Here, we report a family of bacterial actins of unknown function, conserved among the Verrucomicrobiota phylum, which assembles into a unique tubular structure in the presence of ATP. We identified a family of actin homologs, most closely related to MamK (25 to 30% sequence identity) but present in non-magnetotacic bacteria, and therefore presumably with a distinct function. Sequence analysis confirms that it possesses the conserved residues for ATP binding and hydrolysis, and structure prediction confirmed that it likely adopts an actin-like fold. 2d classification suggested that it adopts a rail tracks-like architecture, consisting of two strands rotating on their individual axis (Inset). This prompted us to name this family the Bacterial elongated entwined Rail-like protein (BeeR).

We next used cryo-EM to determine the structure of the BeeR filament, to 3.1 Å resolution. This revealed that it adopts a three-stranded, parallel, right-handed, staggered filament architecture. The diameter of this filament, at ~80 Å, is significantly larger than most other actin-like proteins, and it includes a ~25 Å-wide cavity at its core, responsible for its rail track-like appearance by negative-stain EM. BeeR possesses the canonical actin domains Ia, Ib, IIa, and IIb, with the nucleotide buried between domains Ib and IIb. The longitudinal interface along strands is largely similar to other actin-like filaments, with domains Ib and IIb making extensive contacts with domains IIa of the subunit above. The cross-strand contacts in the BeeR filament are distinct to that of other actin-like filaments. Each protomer interacts with two consecutive subunits of the adjacent strand, as shown on Fig. 2C. Contacts with the top subunit are minimal, with an interface area of ~35 Å2, and consist of a hydrogen bond network between Arg 157 of one subunit and Thr 307 and Gln 310 in the adjacent subunit. In contrast, the contact with the bottom subunit is extensive, forming a contact surface area of ~ 450 Å2, and consists of multiple hydrogen bonds, between Glu 149/Glu 153 and Asn 246 and between Arg 242/Arg 252 and Asn 380. The N-terminal domain, which we identified as a hallmark of the BeeR family is not resolved in our map, supporting its intrinsically disordered nature.

>[12x]MIPASTEKPVPSAAIPANAPNVAVSKPAAPGTRTKTVLVGFDFGTNKSCVLAGTAGATDIAISKIVPTVVGYVKEGIVDGIVAGNRSVLFGDDALQNRLHARLVAPMEHGVIAHPDAARDFVQHLRSLADPSGQAEIRAVVGVPANATEQAREDVRRCAFGIFDRILLIPEPFLAALGYRDDARLGQSNYIDPVVNSLFIDIGGGTSDICLVQGYFPGPDDQISIPFAGDAIDQLLQEELNRTYPNNGLSLHKVREIKEAHGYVGPSRKPLDVKVVIGGKAHTLELGDTLARACNALIDKIYPALTTLIQRASSDSVVTLLQNIIITGGGSQIKGIDTLLQKKLTEDGFESPKVRLAGHDYKRYVALGALKAARAARENQWQVLLG>[4x]CGIVGIAGVMPVNQSIYDALTVLQHRGQDAAGIITIDANNCFRLRKANGLVSDVFEARHMQRLQGNMGIGHVRYPTAGSSSASEA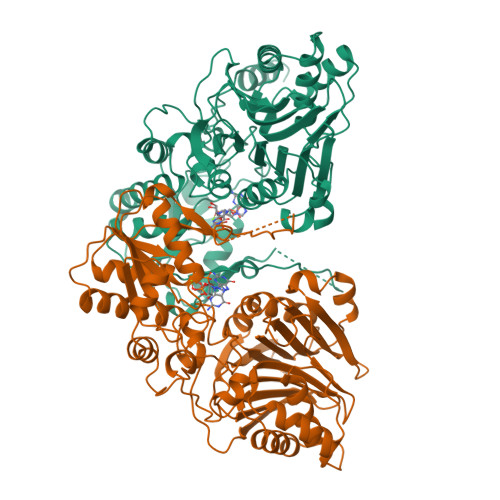QPFYVNSPYGITLAHNGNLTNAHELRKKLFEEKRRHINTTSDSEILLNIFASELDNFRHYPLEADNIFAAIAATNRLIRGAYACVAMIIGHGMVAFRDPNGIRPLVLGKRDIDENRTEYMVASESVALDTLGFDFLRDVAPGEAIYITEEGQLFTRQCADNPVSNPCLFEYVYFARPDSFIDKISVYSARVNMGTKLGEKIAREWEDLDIDVVIPIPETSCDIALEIARILGKPYRQGFVKNRYVGRTFIMPGQQLRRKSVRRKLNANRAEFRDKNVLLVDDSIVRGTTSEQIIEMAREAGAKKVYLASAAPEIRFPNVYGIDMPSATELIAHGREVDEIRQIIGADGLIFQDLNDLIDAVRAENPDIQQFECSVFNGVYVTKDVDQGYLDFLDTLRNDDAKAVQRQNEVENLEMHNEG>[2x]MAQVQPWVDEDLKDS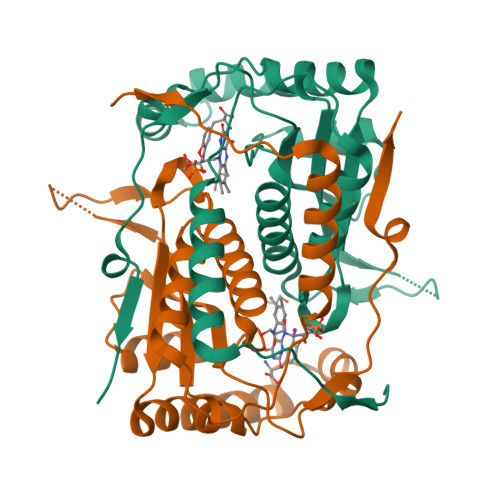TEDLQVEEDAEEWQEAEESVEHIPFSHTRYPEQEMRMRSQEFYELLNKRRSVRFISSEHVPMEVIENVIKAAGTAPSGAHTEPWTFVVVKDPDMKHKIREIIEEEEEINYMKRMGKRWVTDLKKLRTNWIKEYLDTAPVLILIFKQVHGFAANGKKKVHYYNEISVSIACGLLLAALQNAGLVTVTTTPLNCGPRLRVLLGRPSHEKLLVLLPVGYPSRDATVPDLKRKALDQIMVTVHHHHHH> MGALIPSSTLFNIFDFNPKKVRIAFIAVGLRGQTHVENMARRDDVEIVAFADPDPYMVGRAQEILKKNGKKPAKVFGNGNDDYKNMLKDKNIDAVFVSSPWEWHHEHGVAAMKAGKIVGMEVSGAITLEECWDYVKVSEQTGVPLMALENVCYRRDVMAILNMVRKGMFGELVHGTGGYQHDLRPVLFNSGINGKNGDGVEFGEKAFSEAKWRTNHYKNRNGELYPTHGVGPLHTMMDINRGNRLLRLSSFASKARGLHKYIVDKGGESHPNAKVEWKQGDIVTTQIQCHNGETIVLTHDTSLQRPYNLGFKVQGTEGLWEDFGWGEAAQGFIYFEKIMNHSHRWDSSEKWIKEYDHPMWKKHEQKAVGAGHGGMDYFLDNTFVECIKRNEAFP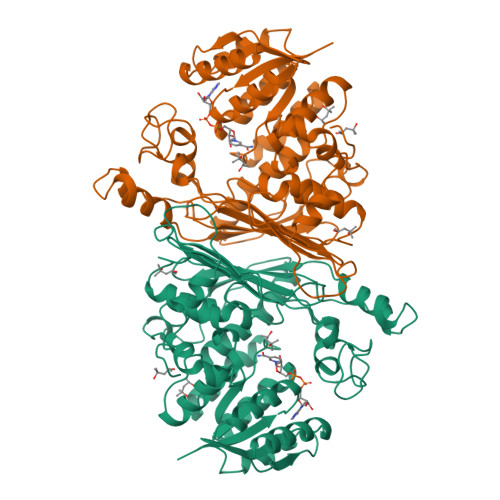LDVYDLATWYSITPLSEKSIAENGAVQEIPDFTNGKWKNAKNTFAINDDY> GSHMEANENILKLKLYRSLGVILDLENDQVLINRKNDGNIDILPLDNNLSDFYKTKYIW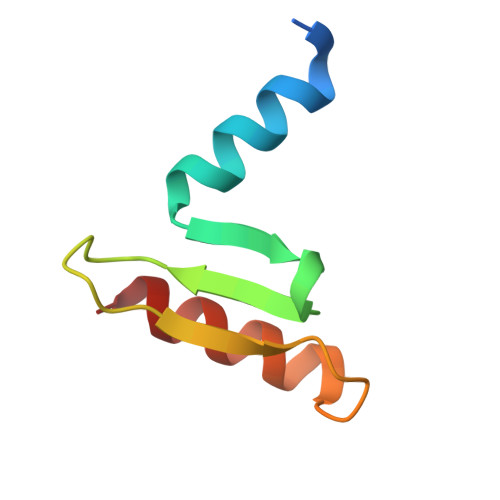ERLGK>MGSHHHHHHSGSMTPILAAEALTYAFPGGVKALDDLSLAVPKGESLAILGPNGAGKSTLLLHLNGTLRPQSGRVLLGGTATGHSRKDLTGWRRRVGLVLQDADDQLFATTVFEDVSFGPLNLGLSEAEARARVEEALAALSISDLRDRPTHMLSGGQKRRVAIAGAVAMRPEVLLLDQPTAGLDLAGTEQLLTLLRGLRAAGMTLVFSTHDVELAAALADRVALFRTGRVLAEGAAEAVLSDRATLAKVALRPPLVIDLALLARDHGLLAPEAPLPKTRDALAAQMAGWTRR[2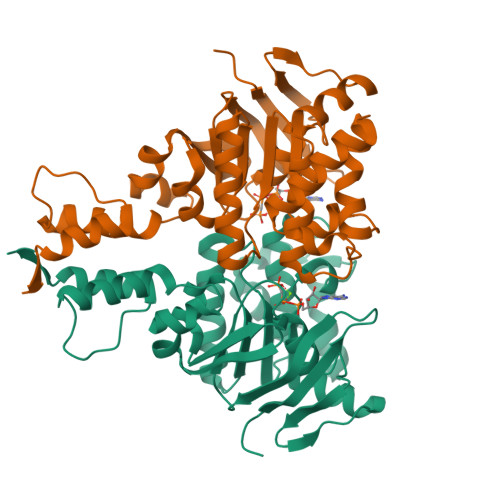x]Using electron cryo-microscopy (cryo-EM) and single particle analysis, we determined the organization of the tail proximal extremity of siphophage T5 that possesses a long flexible tail and solved the structure of its tail terminator protein p142 (TrP142). In siphophages, functional tails are produced after capping of the tail tube by the tail terminator proteins (TrP), of which siphophage λ gpU is the prototype. TrPp142 is resolved as a hexameric ring, interacting with the last tail tube protein TTPpb6 ring. TrPp142 is a 161-residues protein, mainly formed by a four-strand antiparallel β-sheet that lines the lumen of the tube, flanked by two α-helices, and a short loop between β-strands 1 and 2.

We also imaged T5 tails after interaction with E. coli receptor FhuA reconstituted into nanodiscs (Tail-FhuA) with cryo-EM. Image analysis yielded a second 3D map for the proximal extremity of Tail-FhuA, at an average resolution of 4 Å allowing us to build pseudo-atomic models for TrPp142 and TTPpb6. At the resolution of our maps, no conformational change was observed in TrPp142 monomers or hexamer (rmsd 0.43 Å over 156 residues between Tail and Tail-FhuA individual monomers), and neither in TTPpb6. For the latter, it was already shown that the T5 tail tube, formed of a stack of TTPpb6 trimeric rings, does not undergo any conformational changes upon interaction with FhuA and that the signal of the infection is not transmitted from the receptor to the capsid through the tube itself. Because TMPpb2 is expelled during the infection process, the lumen of the tube is empty in Tail-FhuA, which constitutes the only difference between the two EM maps of the tail proximal extremity. By also determining the structure of the T5 tail proximal extremity after interaction with T5 bacterial receptor FhuA, we showed that no conformational changes occur in TrPp142 and confirmed that the infection signal transduction is not carried by the tube itself. TrPs homologous proteins from myophages or tail-like machines also show no conformational change upon infection.

>MDHRTSIAQAMVDRISKQMDGSQPDEYFNNLYGNVSRQTYKFEEIREFPYVAVHIGTETGQYLPSGQQWMFLELPILVYDKEKTDIQEQLEKLVADIKTVIDTGGNLEYTVSKPNGSTFPCEATDMIITSVSTDEGLLAPYGLAEINVTVRYQPPRRSLRR[6x];>[3x]MSLQLLRNTRIFVSTVKTGHNKTNTQEILVQDDISWGQDSNSTDITVNEAGPRPTRGSKRFNDSLNAAEWSFSTYILPYKDKNTSKQIVPDYMLWHALSSGRAINLEGTTGAHNNATNFMVNFKDNSYHELAMLHIYILTDKTWSYIDSCQINQAEVNVDIEDIGRVTWSGNGNQLIPLDEQPFDPDQIGIDDETYMTIQGSYIKNKLTILKIKDMDTNKSYDIPITGGTFTINNNITYLTPNVMSRVTIPIGSFTGAFELTGSLTAYLNDKSLGSMELYKDLIKTLKVVNRFEIALVLGGEYDDERPAAILVAKQAHVNIPTIETDDVLGTSVEFKAIPSDLDAGDEGYLGFSSKYTRTTINNLIVNGDGATDAVTAITVKSAGNVTTLNRSATLQMSVEVTPSSARNKEVTWAITAGDAATINATGLLRADASKTGAVTVEATAKDGSGVKGTKVITVTAGG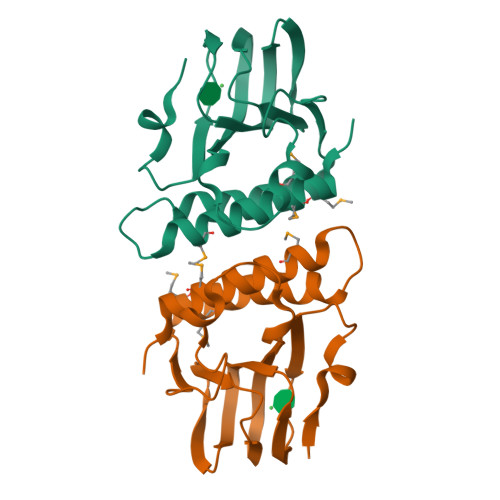>[2x]MAHQLKLLKDDFFASDQQAVAVADRYPQDVFAEHTHDFCELVIVWRGNGLHVLNDRPYRITRGDLFYIHADDKHSYASVNDLVLQNIIYCPERLKLNLDWQGAIPGFNASAGQPHWRLGSMGMAQARQVIGQLEHESSQHVPFANEMAELLFGQLVMLLNRHRYTSDSLPPT>MRGSHHHHHHLVPRGSNVAGLFNNCVACFEYVQLGRHFGRDYERCQLRLDIAKARLSRWGEAVKINDDPRFHSDAPTDKSVQLAKSIVEEILLLFESAQKTSKRYELVADQQDLVVFEDKDMKPIGRALHRRLN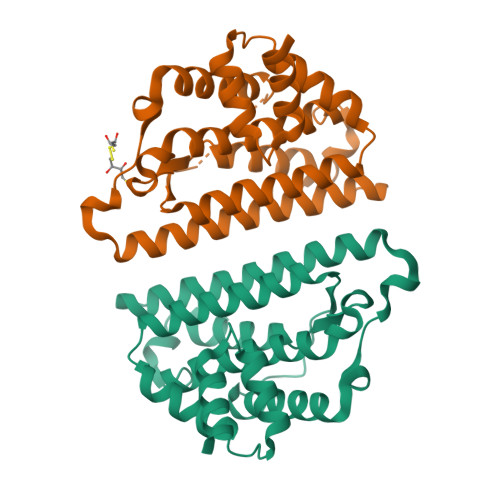DLVSRRQKQTSLAKKTAWALYDGKSLEKIVDQVARFVDELEKAFPIEAVCHKLAEIEIEEVEDEASLTILKDAAGGIDAAMSDAAAQKIDA[2x]>[2x]SQKILQFEDILANTFYREHFGMYMERMDKRALISFWESVEHLKNANKNEIPQLVGEIYQNFFVESKEISVEKSLYKEIQQALVGNKGIEVFYKIQEDVYETLKDRYYPSFIVSDLYEKLLIKEE

One of the most highly conserved sub-families are the SNX proteins with regulator of G-protein signalling (RGS) domains or SNX-RGS proteins. Other well-characterised family members include Mdm1 from Saccharomyces cerevisiae and Snazarus (Snz) from Drosophila melanogaster. These proteins have relatively low sequence similarity across homologues and across species but share a conserved architecture with an N-terminal hydrophobic membrane anchor, and a central RGS domain and PX domain (except for SNX19 orthologues which lack the RGS domain). The N-terminal membrane anchor mediates localisation to the endoplasmic reticulum (ER), and the proteins typically localise to sites of new lipid droplet synthesis and can enhance membrane tethering of the ER to other membrane compartments via their PX domains including the vacuole in yeast, the plasma membrane in Drosophila and endolysosomal compartments in mammalian cells. The precise function of the SNX-RGS proteins is still unclear although their mutation or depletion has significant impacts on cellular physiology, particularly with respect to lipid homeostasis and endolysosomal function.

Here we have also solved the structure of the human SNX25 RGS domain by X-ray crystallography in two crystal forms. Here we have solved the crystal structure of the human SNX25 RGS domain, revealing a typical α-helical RGS fold. We next investigated how similar the experimentally determined SNX25 RGS domain was to the predicted structure from the AlphaFold2 database. The structure predicted by AlphaFold2 is remarkably close to the SNX25 crystal structure, with an overall root-mean-squared-deviation (RMSD) of 0.8 Å over 107 Cα atoms. Side chain conformations in general were likewise closely aligned between the experimental and predicted structures. The predicted structures of the human SNX13 and SNX14 RGS domains from the AlphaFold2 database are generally similar to the experimental SNX25 RGS domain structure as expected, but with some notable differences. In general, the three domains have relatively low sequence homology, and this is reflected for example in a significantly longer α3-α4 extension in SNX13 compared to the other two proteins and. Overall, these comparisons confirm that the AlphaFold2 predictions of selected SNX-RGS domains are accurate models comparable to their known experimental structures, including the RGS domain of SNX25 for which no detailed structural information was available prior to this study.>[2x]GSAE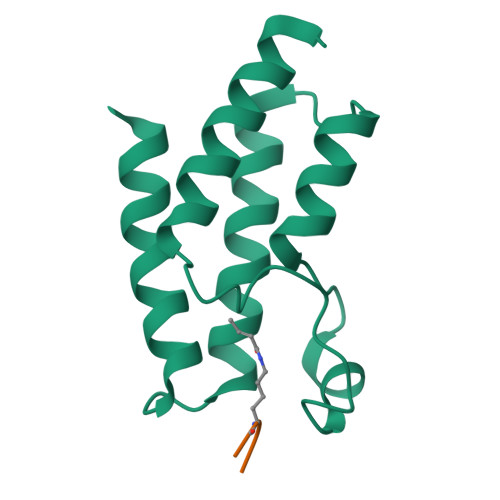NESTPIQQLLEHFLRQLQRKDPHGFFAFPVTDAIAPGYSMIIKHPMDFGTMKDKIVANEYKSVTEFKADFKLMCDNAMTYNRPDTVYYKLAKKILHAGFKMMSK;>SGRGXGGXGLG[2x]>[3x]GSHMGQSLRTLQGHQSAVTSLQFNDNIVVSGSDDSTVKVWDIKTGQSLRTLQGHQSAVTSLQFNDNIVVSGSDDSTVKVWDIKTGQSLRTLQGHQSAVTSLQFNDNIVVSGSDDSTVKVWDIKTGQSLRTLQGHQSAVTSLQFNDNIVVSGSDDSTVKVWDIKTGQSLRTLQGHQSAVTSLQFNDNIVVSGSDDSTVKVWDIKTGQSLRTLQGHQSAVTSLQFNDNIVVSGSDDSTVKVWDIKTGQSLRTLQGHQSAVTSLQFNDNIVVSGSDDSTVKVWDIKTGQSLRTLQGHQSAVTSLQFNDNIVVSGSDDSTVKVWDIKGS

WD40 proteins are a subfamily of propeller proteins with no intrinsic enzymatic activity, but their stable, modular architecture and versatile surface have allowed evolution to adapt them to many vital roles. By computationally reverse-engineering the duplication, fusion and diversification events in the evolutionary history of a WD40 protein, a perfectly symmetrical homologue called Tako8 was made. A different computational approach was employed to redesign Tako8 to create Ika8, a fourfold-symmetrical protein in which neighbouring blades carry compensating charges. Tako and Ika are the first successfully designed eight-bladed WD40-repeat proteins for which structures have been confirmed crystallographically.

The high symmetry of the Tako protein is evident from the crystal structure, and determination of the space group proved challenging (Tako8 crystal No. 2). In both crystal forms the Tako8 molecules show a conserved interaction at the top side where two proteins meet face to face. The crystal-packing interaction is mediated by a hydrogen-bonding pattern with eightfold symmetry. The difference between the two crystal forms arises from different water-mediated interactions at the outer rim of the toroid. The individual repeats of the Tako8 protein can be perfectly aligned. In comparison, only the alternating repeats of the Ika proteins can be superposed, in contrast to the template structure where the overlap of the individual blades is much poorer. The symmetry is also visible in the electrostatic potential map, where eightfold and fourfold symmetry can be observed for Tako8 and Ika8, respectively, with the exception of small differences owing to crystal-packing inter­actions; such charge symmetry is absent from the template protein. Tako8 was found to have highest stability around pH 8, but to be extremely unstable in the absence of salt. Increasing the salt concentration led to increased stability over the tested pH range.BETA-6-HYDROXY-1,4,5,6-TETRAHYDRONICOTINAMIDE ADENINE DINUCLEOTIDE 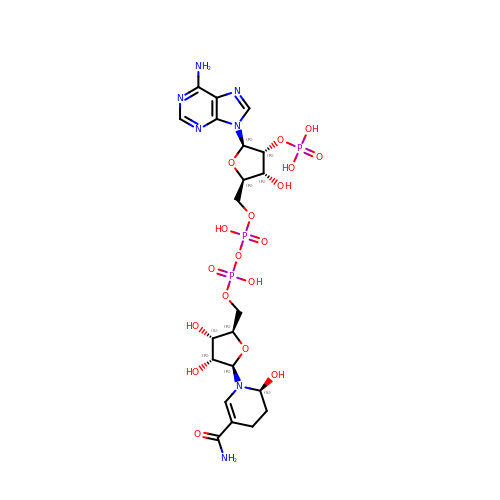PHOSPHATE | C21 H32 N7 O18 P3 | SZKXTJUOKARGIY-VPHRTNKSSA-N(2R,6S,12Z,13aS,14aR,16aS)-6-[(tert-butoxycarbonyl)amino]-14a-[(cyclopropylsulfonyl)carbamoyl]-5,16-dioxo-1,2,3,5,6,7,8,9,10,11,13a,14,14a,15,16,16a-hexadecahydrocyclopropa[e]pyrrolo[1,2-a][1,4]diazacyclopentadecin-2-yl 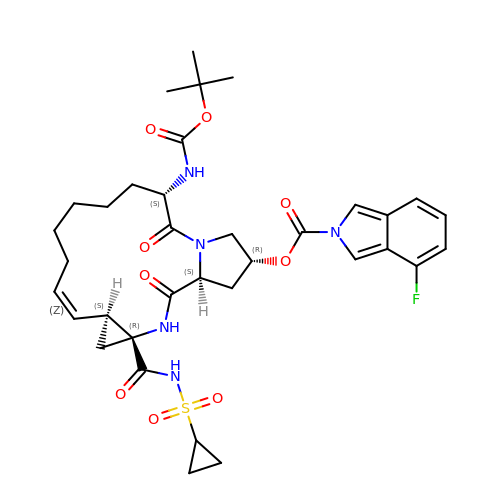4-fluoro-2H-isoindole-2-carboxylate | C35 H44 F N5 O9 S | YUWURHBDLJOUAP-JSZLBQEHSA-N> XQIAAIKXAIAAIKQQIAAIKEAI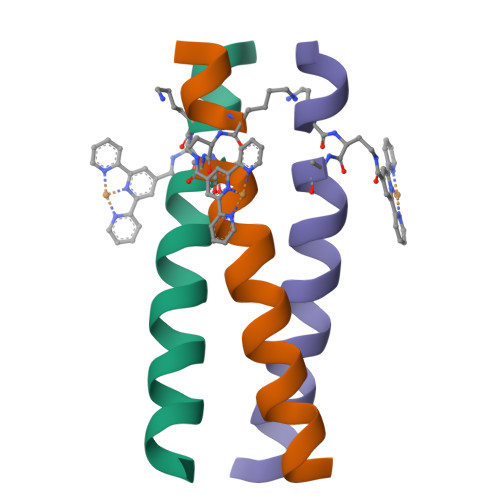AAIKQX> KQIADSLSIPPVKAGAKQLPMPSVSGAQIKLLGADYEQLVNSKGKIAPVISDTPVNVSFKVTKDGKEAVSKDYEIMLQAPQAAQGNPKPRIIPEILQWKGGQGEYKLGNTVTIACPDKELGKLFAADMEDVLGKKVKLVAPGAKADISLSLLKGGNLGREGYRLQIARDGVRLGAAAPTGLFWGTRTLLQMLRQTPGSVPCGTAVDFPRYQLRGFMLDVARTPYPLSYLKDVIRTMAWYKMNDLHLVINNNYIFHEHYVDNGHDPFKESYAAFRLESKMKGKDGTPLTARDLFYTKKEFADLVSYARKYGVNIVPEFDTPGHALSFTRLRPDLIYKGPMNHEKRRCEMLDAANPETIDLVSKVFDEYMLKDPKLGRPVFADCGVVHVGADEFYGDKEDYRHFANAVLTHALKRGYTPRIWGSLSAKPGKTPVVSKGVQMNLWSTGWMKAWEAVNQGYD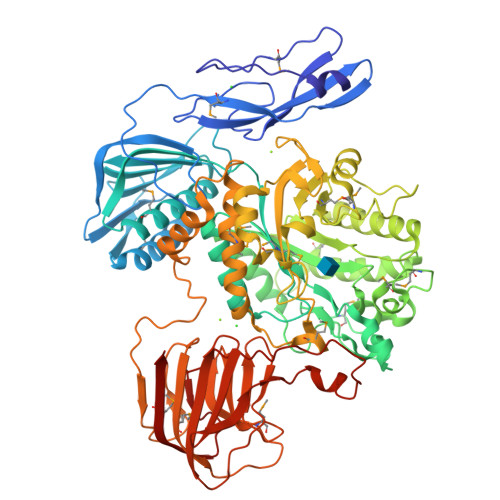VINTNDGALYIVPFAGYYRMDRNHKGLYNNWIPNRIGNETLPSGHPQLLGGTFAVWNDETDIMHTGYAPYDIWGIISGSMDVLSQKLWGTAKAPDTFEQHRELVSSIGNAPRTNPLHKWKDSQPLTVKPSSLPQKLDKPALGPNYRLTMELELTAAPEGKEQVLLAAPEGELLAVMKDGTVGFRRDDSLEFSFGAKLPVGKKVKVEIVGEPEKTSLLLDGEPAGTAVLKNFSDKSKDFSDKFKHRPKVHRSTFILPLKELGSSFQGKVFHMNVQPL> MEPSSKKLTGRLMLAVGGAVLGSLQFGYNTGVINAPQKVIEEFYNQTWVHRYGESILPTTLTTLWSLSVAIFSVGGMIGSFSVGLFVNRFGRRNSMLMMNLLAFVSAVLMGFSKLGKSFEMLILGRFIIGVYCGLTTGFVPMYVGEVSPTALRGALGTLHQLGIVVGILIAQVFGLDSIMGNKDLWPLLLSIIFIPALLQCIVLPFCPESPRFLLINRNEENRAKSVLKKLRGTADVTHDLQEMKEESRQMMREKKVTILELFRSPAYRQPILIAVVLQLSQQLSGINAVFYYSTSIFEKAGVQQPVYATIGSGIVNTAFTVVSLFVVERAGRRTLHLIGLAGMAGCAILMTIALALLEQLPWMSYLSIVAIFGFVAFFEVGPGPIPWFIVAELFSQGPRPAAIAVAGFSNWTSNFIVGMCFQYVEQLCGPYVFIIFTVLLVLFFIFTYFKVPETKGRTFDEIASGFRQGGASQSDKTPEELFHPLGADSQVLVPR

The human glucose transporters GLUT1 and GLUT3 have a central role in glucose uptake as canonical members of the Sugar Porter (SP) family. GLUTs belong to the Sugar Porter (SP) family, which as the largest branch of the Major Facilitator Superfamily (MFS), is found in all kingdoms of life. MFS proteins share a common fold comprising of 12 transmembrane helices (M1–M12) with a twofold pseudo-symmetry between the N-domain (M1-6) and the C-domain (M7-12). SP proteins alternate between inward facing and outward facing conformations with respect to the central substrate binding site, and the transition between these two states define sugar transport.

We subsequently solved the crystal structure of human GLUT1 to 2.4 Å resolution (Rfree 22.9%). The overall structure adopts an inward-open conformation that is almost identical to the 3.2 Å model published previously (RMSD(CA) 0.4 Å). The structure consists of residues 9–455 (of 492 residues total) and contains the N-domain, the cytosolic ICH domain (ICH1-ICH4), and the C-domain. In our maps, we clearly observe an NG molecule in the central sugar-binding pocket in the N-domain, despite having a sixfold molar excess of glucose present (40 versus 6.5 mM). Residues from the C-domain coordinate the glucose headgroup, with seven polar interactions established through residues from M7, M8, and M10. Next to the glucose headgroup, we also observe an additional tubular density close to the binding site that fits with a polyethylene glycol (PEG) molecule, derived from the experimental setup. The position of this PEG molecule matches previously identified inhibitor positions in GLUT1. By replacing Cl− with Br− in the crystal it is possible to search for anomalous density peaks to identify bromide ion positions which will reveal the original chloride position in the previous dataset. This experiment lead to a single strong anomalous peak (7.3 sigma) at the position of the spherical density in the native dataset, allowing us to unequivocally identify this peak as a Cl− ion positioned between the SP and A motif in the N-domain. The chloride ion is coordinated by several residues of the A-motif in the N-domain including the backbones of Arg92, Arg93, as well as Glu209 from the SP motif, with hydrogen bonds ranging in distance from 3.2 to 3.6 Å. Indeed, the D-glucopyranoside headgroup in this “secondary site” establishes polar interactions with Arg93, Asn94, Glu209, Arg218, and Arg223 from both the N-domain SP motif, ICH1-2 and M3 residues.>[2x]AEPNLYGRYEWVSLPELDRTLQAKMDTGAYTSSLSAKDIELFQRDGEEWVRFRLATKEADGSVFEHKLARIGKIKNRADNRSGEDEDEDRLSERPVIDLQV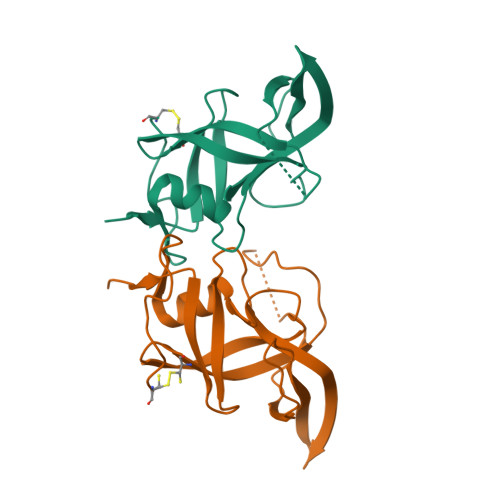CLGGAMKTIEVNLTDRSAFNYPFLMGTKGLRKFHVAVDPSERFVADKPTCK>[2x]LQSGSKFVKIKPVNNLR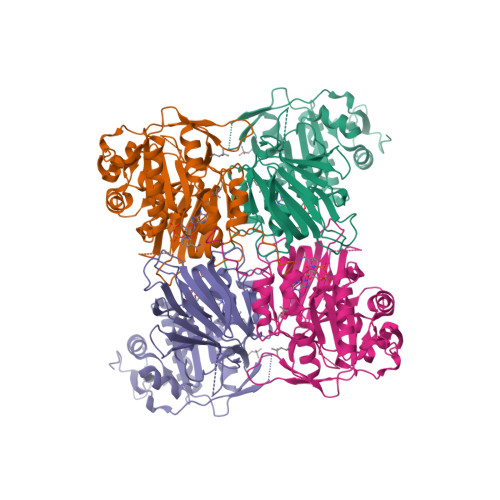SSSSADFVSPPNSKLQSLIWQNPLQNVYITKKPWTPSTREAMVEFITHLHESYPEVNVIVQPDVAEEISQDFKSPLENDPNRPHILYTGPEQDIVNRTDLLVTLGGDGTILHGVSMFGNTQVPPVLAFALGTLGFLSPFDFKEHKKVFQEVISSRAKCLHRTRLECHLKKKDSNSSIVTHAMNDIFLHRGNSPHLTNLDIFIDGEFLTRTTADGVALATPTGSTAYSLSAGGSIVSPLVPAILMTPICPRSLSFRPLILPHSSHIRIKIGSKLNQKPVNSVVKLSVDGIPQQDLDVGDEIYVINEVGTIYIDGTQLPTTRKTENDFNNSKKPKRSGIYCVAKTENDWIRGINELLGFNSSFRLTKRQTDND>[2x]GSHMGQNDLVKTLRMNYLFDFYQSLLTNKQRNYLELFYLEDYSLSEIADT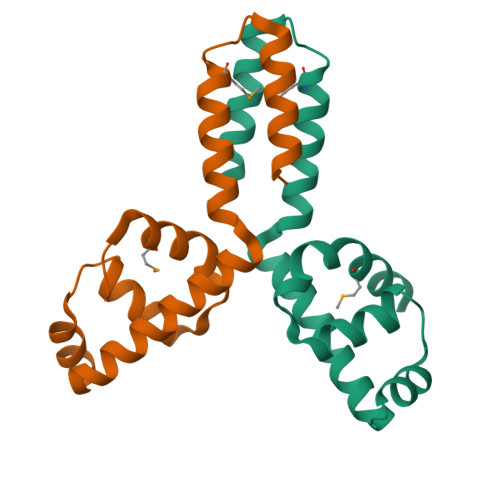FNVSRQAVYDNIRRTGDLVEDYEKKLELYQKFEQRREIYDEMKQHLSNPEQIQRYIQQLEDLE> GPDSMT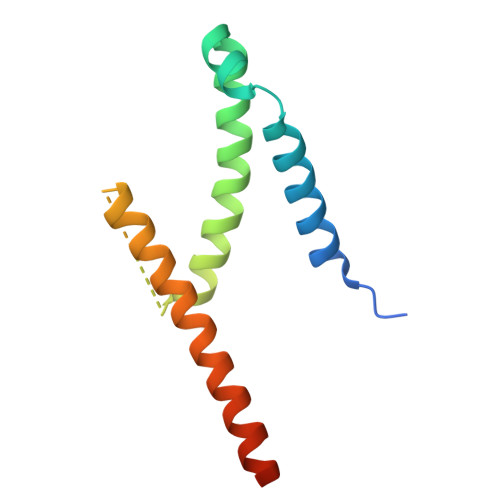SENPDVLLSRVINVVRAASSLASQDVDFYKNLDRGFSKDLKSKADKLADMANEIILSIDEHHESFELKEEDISDLWNNFGNIMDNLLEMSDHSLDKLNCAINSKSRGSD>EEIRPKEVYLDRKLLTLEDKELGSGNFGTVKKGYYQMKKVVKTVAVKILKNEANDPALKDELLAEANVMQQLDNPYIVRMIGICEAESWMLVMEMAELGPLNKYLQQNRHVKDKNIIELVHQVSMGMKYLEESNFVHRDLAARNVLLVTQHYAKISDFGLSKALRADENYYKAQTHGKWPVKWYAPECINYYKFSSKSDVWSFGVLMWEAFSYGQKPYRGMKGSEVTAMLEKGERMGCPAGCPREMYDLMNLCWTYDVENR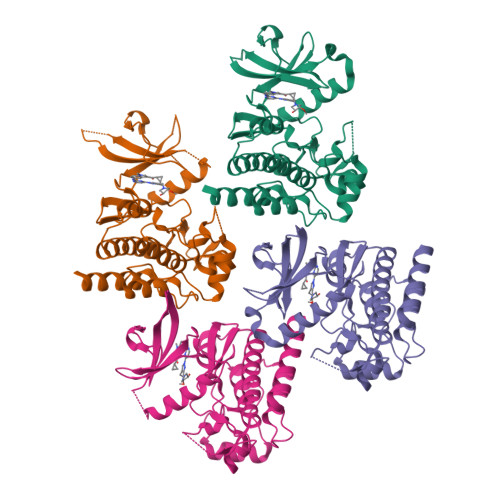PGFAAVELRLRNYYYDVVNLEHHHHHHHH[4x]> MADLFKQFRLGKDYGNNSTIAQVPIDEGLQANIKKIEQDNKEYQDLTKSLYGQQQAYAEPFIEMMDTNPEFRDKRSYMKNEHNLHDVLKKFGNNPILNAIILTRSNQVAMYCQPARYSEKGLGFEVRLRDLDAEPGRKEKEEMKRIEDFIVNTGKDKDVDRDSFQTFCKKIVRDTYIYDQVNFEKVFNKNNKTKLEKFIAVDPSTIFYATDKKGKIIKGGKRFVQVVDKRVVASFTSRELAMGIRNPRTELSSSGYGLSEVEIAMKEFIAYNNTESFNDRFFSHGGTTRGILQIRSDQQQSQHALEN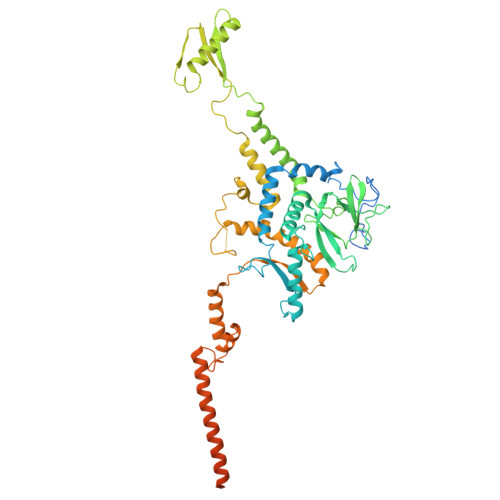FKREWKSSLSGINGSWQIPVVMADDIKFVNMTPTANDMQFEKWLNYLINIISALYGIDPAEIGFPNRGGATGSKGGSTLNEADPGKKQQQSQNKGLQPLLRFIEDLVNRHIISEYGDKYTFQFVGGDTKSATDKLNILKLETQIFKTVNEAREEQGKKPIEGGDIILDASFLQGTAQLQQDKQYNDGKQKERLQMMMSLLEGDNDDSEEGQSTDSSNDDKEIGTDAQIKGDDNVYRTQTSNKGQGRKGEKSSDFKH The p85α protein serves as a regulatory protein for both p110α and PTEN. The p85α protein contains 5 domains, an SH3 (Src Homology 3) domain capable of binding proline-rich sequences, a BH (break-point cluster region homology) domain, an N-terminal SH2 (Src Homology 2) domain (nSH2), an inter-SH2 domain (iSH2) and a C-terminal SH2 domain (cSH2). Importantly, the BH domain of p85α, either alone or together with the SH3 domain, also mediates binding to PTEN via a distinct interaction that does not compete with Rab5 binding. The p85α protein can dimerize and these dimers associate with PTEN, protecting it from ubiquitination and proteasomal degradation to stabilize PTEN levels.

A unique feature we noticed in the bovine p85α BH domain structure that was not described in the previous paper, was clear electron density for two sulfate ions near residues K224, R228, H234, W237, and Q241. The residues involved in coordinating the pair of sulfate ions within the bovine p85α BH domain are conserved in the human protein and they adopt similar positions within the structure, suggesting it may also contain a novel binding site. We generated, crystalized and determined the structure of the p85α-BH-R228E protein (2.4 Å), containing a mutation in a potential sulfate binding site residue. In this crystal structure, one of the sulfate ions was clearly absent, and the remaining sulfate ion reoriented itself within the site. No other major structural differences were observed. This result is consistent with R228 contributing to sulfate binding. We recognize that sulfate binding to Arg is very common in proteins crystallized from ammonium or lithium sulfate solutions, but the distance between the two sulfate positions (7.1 Å) is similar to that of the two PO4 groups (6.8 Å) in inositol 1,3,4,5-tetrakisphosphate, raising the intriguing possibility that this surface may recognize phospholipid head groups. The docking model predicts that p85α-R228 makes contacts with peptide backbone main-chains C250 and D252 within the PTEN C2 domain. Both the p85α-K225E and p85α-R228E mutants showed significant reductions in PTEN binding without altering their ability to stimulate PTEN lipid phosphatase activity, whereas the p85α-Q221E mutant behaved like the wild type p85α protein. Several of the p85α BH domain residues that can bind a pair of sulfate ions are also involved in mediating interactions with PTEN, suggesting that if phosphorylated lipids bind to the p85α BH domain at this location, binding of lipid and PTEN would be mutually exclusive.

>[2x]GPLGSTEADSQQASTLPDLAEQFAPPDVAPPLLIKLVEAIEKKGLECSTLYRTQSSSNPAELRQLLDCDTASLDLEMFDVHVLADAFKRYLLDLPNPVIPVAVSSELISLAPEVQSSEEYIQLLKKLIESPSIPHQYWLTLQYLLKHFFKLSQTSSKNLLNARVLSELFSPLLFRFPAASSENTEHLIKIIEILISTEWNERQPAPALPPKPPKPTTVAN>GPGSMTTTDDRYAGVLRLDGKRALITGATKGIGADIARAFAAAGARLVLSGRDVSELDAARRALGEQ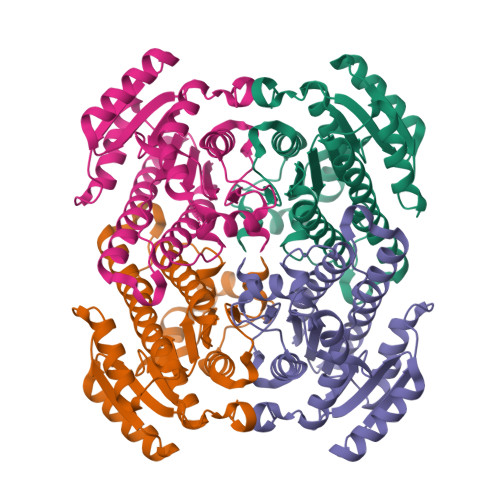FGTDVHTVAIDLAEPDAPAELARRAAEAFGGLDVLVNNAGISHPQPVVDTDPQLFDATIAVNLRAPALLASAVGKAMVAAGEGGAIITVASAAALAPLPDHYAYCTSKAGLVMATKVLARELGPHGIRANSVCPTVVLTEMGQRVWGDEAKSAPMIARIPLGRFAVPHEVSDAVVWLASDAASMINGVDIPVDGGYTMG[8x]> 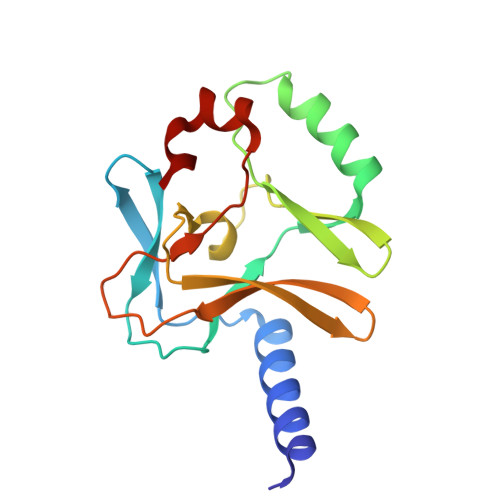KSKAELQSEERKRIDELIESGKEEGMKIDLIDGKGRGVIATKQFSRGDFVVEYHGDLIEITDAKKREALYAQDPSTGCYMYYFQYLSKTYCVDATRETNRLGRLINHSKSGNCQTKLHDIDGVPHLILIASRDIAAGEELLYDYGDRSKASIEAHPWLKH> AH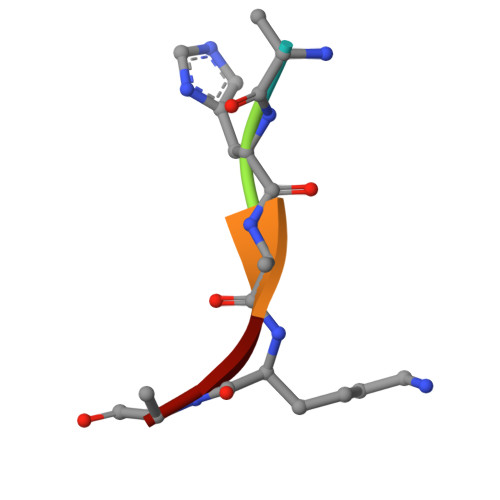AKA>MKEDQVVAEEPGFQDEEESLFQDIDLLQKHGINVADIKKLKSVGICTIKGIQMTTRRALCNVKGLSEAKVDKIKEAANKLIEPGFLTAFEYSEKRKMVFHITTGSQEFDKLLGGGIESMAITEAFGEFRTGKTQLSHTLCVTAQLPGAGGYPGGKIIFIDTENTFRPDRLRDIADRFNVDHDAVLDNVLYARAYTSEHQMELLDYVAAKFHEEAGIFKLLIIDSIMALFRVDFSGRGELAERQQKLAQMLSRLQKISEEYNVAVFVTNQMTADPGATMTFQADPKKPIGGHILAHAST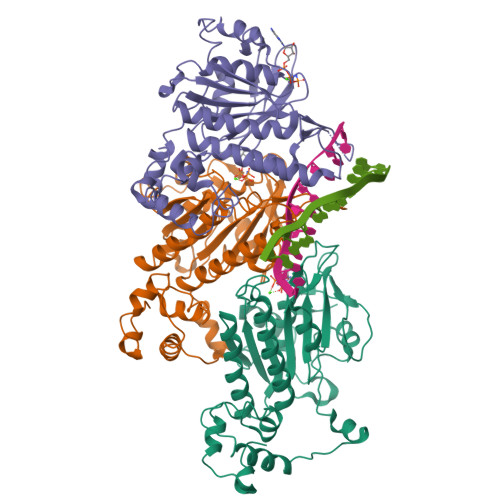TRISLRKGRGELRIAKIYDSPEMPENEATFAITAGGIGDAKE[3x]> GAMEADLSEPFSLTEVQTAYMLGRNPQFELSGISPQTYFEYETELDIARLSRSFQKVIQRHPMLRAVILPEGKQQILRDVPEYEIEVESLVSMPPEKQAARLREERSRMIDHVFPLGQWPLFELKAFQLQEHTYLLCFRYDALLMDGASMNLVGQDLMHYYHQPDAQLPPLSFTFQDYMHIYDDMKRGTEYETAKAYWTNKLPDFPPAPSLLLAKDPAEIGTPNFQSLTTIITKDKWLKLRRLAQDKQVTPSALLCTVYGEVLAFWSNQRRLAINLTVFNRYPVHDEVEQIVGDFTSLILLDMDMDQKQPFFTKVEQTQSTLLDGLEHRHYDGVEFIRDYTRYHQMRPKAVMPIVFTSMLAGAGAFAWEEIGSLRHIHARTPQVYLDNVVIEKNGELLVSWNYVEELFDAEVMESMFTQFVELLDQLVEQGDINPLRISQKDYALIDQYNATAEPIPAATLHQLFIDQAQRTPDQVAVVFEQEWLTYSELDQRSNQVARFLQSRGIGRGDRVGVLA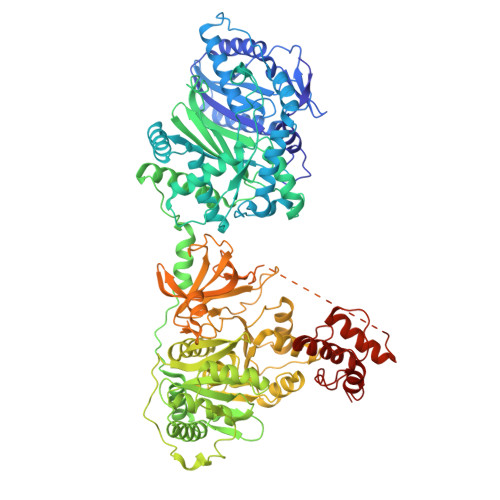KRQVETIINLMAVLKAGAAYVPIDPDHPYERQTYILENSSCKILLDSDLYETMEISSYADGDLTPVAEPEDTAYVIYTSGSTGRPKGVIITHQAASNTIQDINRKFEVNEEDRIIGISSMCFDLSVYDIFGTLSAGATLVMIRDPRDMRELVRTVERRGITIWNTVPAIMDLALDHVGSHFENISLRLVLLSGDWIPLPLPAKINRHFPVADVISLGGATEASIWSIYWPIEQVEANWKSIPYGKPLANQTYYVLNYDQKMCPVGVIGDLYIGGAGLAQGYLNDDQKTKDAFIMHPEFGPIYKTGDCGRMRPEGYIEFLGRQDYQVKIQGYRVELEEISHCLLTYPDVDQAVVIDQTDERGMKFLVGYVVAQQEIDEKALRKHLMEHLPEYMIPAHLVHLEQLPLTPNGKLDRKALPVPKKQRNAEKFVAPQAGLEKILASVWQEVLNVEQIGANDHFFALGGDSIKAIQVSARLFVQGYHLDTKSLFEFPVLRDVARTIKKLAAAENLFY> SLIQFETLIMKVAKKSGMFWYSNYGCYCGWGGQGRPQDATDRCCFVHDCCYGKVTGCDPKMDVYSFSEENGDIVCGGDDPCKKEICECDRAAAICFRDNLTLYNDK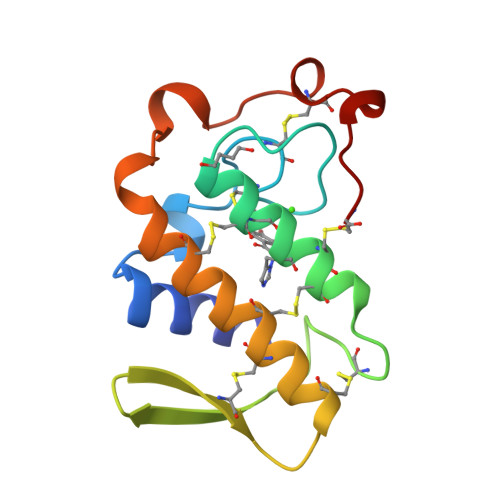KYWAFGAKNCPQEESEPC> GPLGSDHVLHVTFPKEWKTSDLYQLFSAFGNIQISWIDDTSAFVSLSQPEQVKIAVNTSKYAESYRIQTYA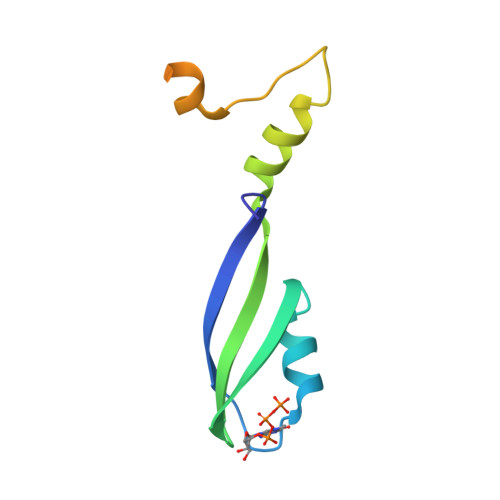EYMGRKQEEKQIKRKWTEDSWKEADSKRLN>CGACGATCGT[2x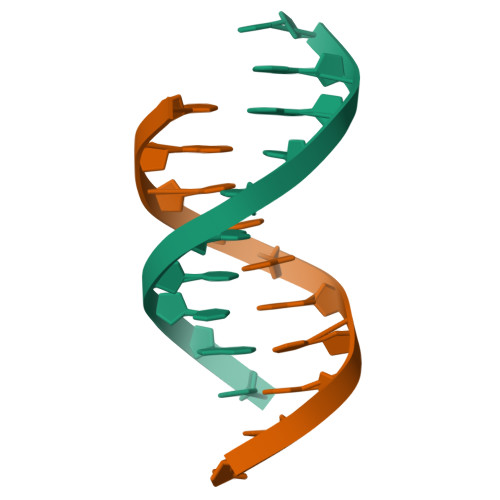]Beta-1,4-galactosyltransferase 1 (B4GalT1; EC 2.4.1.38) is a family 7 glycosyltransferase residing in the trans Golgi. In the presence of manganese, it transfers a galactose moiety (Gal) from UDP-galactose (UDP-Gal) to an N-acetylglucosamine (GlcNAc) residue, with the formation of a β1–4 linkage. B4GalT1 possesses a type II membrane protein topology, with a short N-terminal cytoplasmic tail and an α-helical transmembrane domain responsible for Golgi localization, a stem domain (amino acids 45–125), that is believed to be mostly disordered and whose function is still unknown, and a globular catalytic domain (amino acids 126–398) carrying the sugar transfer activity. Previous structure-function studies of the catalytic domain of B4GalT1 by x-ray crystallography revealed that the enzyme undergoes conformational changes upon substrate binding and during its catalytic cycle.

The closed structure shows two molecules per asymmetric unit, with no significant conformation difference between the two chains. Despite the absence of the lid in this structure, the position of the Trp loop (amino acids 308–311), with Trp310 facing the inside of the catalytic pocket, clearly indicates the presence of the closed conformation. In the closed structure, we observe that loop1 is displaced deeper towards the catalytic pocket than in the open one, with an RMSD ≈ 6–10 Å. Specifically, the one-turn α-helix usually formed by residues 274–277 in the open conformation becomes a β-turn in the closed conformation (arrow a) and residues 280–284 transform from a random coil in the open conformation to a one-turn α-helix in the closed conformation (arrow b). The observed position of loop1 in the closed structure is also such that the lid cannot be in the open conformation because of steric hindrance. There is a symmetrical pair of salt bridges between Glu313 and Arg330, which lie at the rim of the dimer interface. Between them reside hydrophobic contacts, which mostly maintain the dimerization interface: residues from loop1 (Val271, Gly277, Phe278 and Tyr285) and close to the Trp loop (Phe318, Val322 and Phe323). In the closed dimer of the wild-type B4GalT1, the H343 active site residues are 35.5 Å apart. The active sites are slightly tilted relative to each other and there is sufficient space for reaction to occur. The homodimer structure solved here most closely mimics the one that normally exists in the ER, or alternatively, in the Golgi in cells overexpressing only one of the players needed for heteromer formation.

>[2x]SLPACPEESPLLVGPMLIEFNMPVDLELVAKQNPNVKMGGRYAPRDCVSPHKVAIIIPFRNRQEHLKYWLYYLHPVLQRQQLDYGIYVINQAGDTIFNRAKLLNVGFQEALKDYDYTCFVFSDVDLIPMNDHNAYRCFSQPRHISVAMDKFGFSLPYVQYFGGVSALSKQQFLTINGFPNNYWGWGGEDDDIFNRLVFRGMSISRPNAVVGRCRMIRHSRDKKNEPNPQRFDRIAHTKETMLSDGLNSLTYQVLDVQRYPLYTQITVDIGTPS>[4x]GSGGGMFGAFVSHRLWSDSGCTTTCITNSIANYVAFGEQIGFPFKSAQVFIAGPRKAVINIQEDDKVELLKMIVKHNLWVVAHGTYLDVPWSRRSAFVTHFIQQELLICKEVGIKGLVLHLGAVEPELIVEGLKKIKPVEGVVIYLETPHNKHHTYKYSTMEQIKELFLRIRNTRLKQIGLCIDTAHIWSSGVNISSYNDAGQWLRSLENIHSVIPPSHIMFHLNDAATECGSGIDRHASLFEGMIWKSYSHKIKQSGLYCFVEYITRHQCPAILERNLGSSMQLQTALTAEFTTLKSLLK

ASFV AP endonuclease (AsfvAP) catalyzes DNA cleavage reaction at the abasic site and is a key enzyme of ASFV base excision repair (BER) system. AsfvAP belongs to the class II AP endonuclease family; it mainly catalyzes DNA cleavage reaction at the 5′ side of abasic site (AP), generating 3′-OH group and 5′-deoxyribose phosphate (dRP). AsfvAP is of α/β fold in nature; the β-strands form one β-barrel in the center, surrounded by α-helices at the outer side. AsfvAP possesses many unique structural features, including one narrower nucleotide-binding pocket at the active site, the C16–C20 disulfide bond-containing region, and histidine-rich loop.

To unravel the molecular basis underlying substrate binding and cleavage by AsfvAP, we performed crystallographic studies and solved two complex structures of AsfvAP, AsfvAP/DNA-1, and AsfvAP/DNA-2. Both DNA-1 (5′-GCAGCGTCCFCGACGAGG-3′ and 3′-CGTCGCAGGGGCTGCTCC-5′) and DNA-2 (5′-GCAGCGTCACCGACGAAA-3′ and 3′-CGTCGCAGGGGCTGCTCC-5′) are 18-bp dsDNAs, containing one abasic site and one A:G mispair in the middle, respectively. In the AsfvAP/DNA-2 structure, each DNA was bound by two AsfvAP molecules, but the DNA did not interact with any R1 residues. Cys16 could undergo subtle conformational changes, whereas the conformation of the neighboring α-turn and Cys20 of R1 were well fixed in AsfvAP/DNA-1 and AsfvAP/DNA-2 complexes. As revealed by our AsfvAP/DNA-2 structure, AsfvAP has no NIR activity against A:G mispair. The in vitro DNA cleavage assays showed that AsfvAP had no NIR activity against any regular mispairs embedded in the middle of the substrates. AsfvAP does not recognize and cleave the mispairs embedded in the middle of the DNA duplex, but it is able to remove the nucleotides (either paired or mispaired) from the 3′ end or nick site of the DNAs in the absence of abasic sites. Rather than substrate-bound or product-bound state, structural superposition suggested that our AsfvAP/DNA-2 complex may represent one product-releasing state.> ENLYFQGHM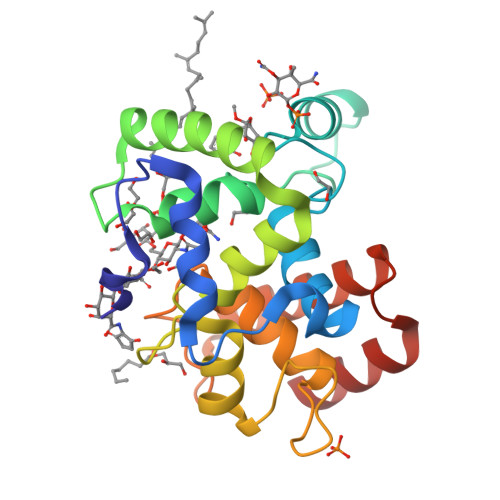DNVDELRKIENKSSFVSADNMPEYVKGAFISMQDERFYNHHGFDLKGTTRALFSTISDRDVQGGSTITQQVVKNYFYDNDRSFTRKVKELFVAHRVEKQYNKNEILSFYLNNIYFGDNQYTLEGAANHYFGTTVNKNSTTMSHITVLQSAILASKVNAPSVYNINNMSENFTQRVSTNLEKMKQQNYINETQYQQAMSQLN~{N}-ethyl-4-oxidanyl-2-oxidanylidene-1~{H}-1,7-naphthyridine-3-carboxamide | C11 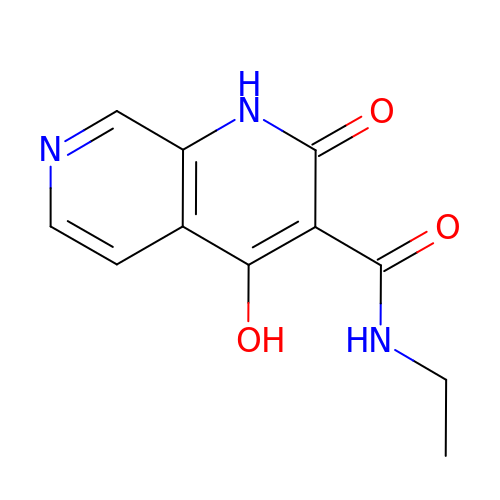H11 N3 O3 | RTMUDFJHLBNEDM-UHFFFAOYSA-N> GAMESKKRQWALEDFEIGRPLGK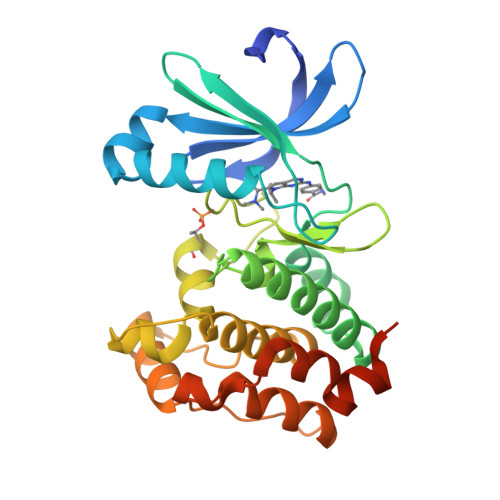GKFGNVYLAREKQSKFILALKVLFKAQLEKAGVEHQLRREVEIQSHLRHPNILRLYGYFHDATRVYLILEYAPLGTVYRELQKLSKFDEQRTATYITELANALSYCHSKRVIHRDIKPENLLLGSAGELKIADFGWSVHAPSSRRTTLAGTLDYLPPEMIEGRMHDEKVDLWSLGVLCYEFLVGKPPFEANTYQETYKRISRVEFTFPDFVTEGARDLISRLLKHNPSQRPMLREVLEHPWITANSSKPSNSQNKESASKQS> MEELLMSLKLKALYPLTGGYNRHSINPFYEELVRPTEIKGLWRWWNRVLFNTLAYSTKGKLYTYESIDRLFEDVFGSENKKSAVRLEVITDEGNDNRFELSYVELDKVIDCLRNYKRKVSLDFIDNTLIAEIEGSTKIPISFKSNLDIDKIIKDLVHNNKLLSFELLGFKSVEIDATKISDKKILKEILRDLITNYLEYFNIKQEVTFTLNIYLDKSREHKQNFEDKLKFALYSLLVFILLGGIGRKTSRGFGSLSIIDVKCYDNSICKKIEDLAKNFLKISSGNELKSKIESILDCIKNSCIDTLYIENNILSEIDPKKNVV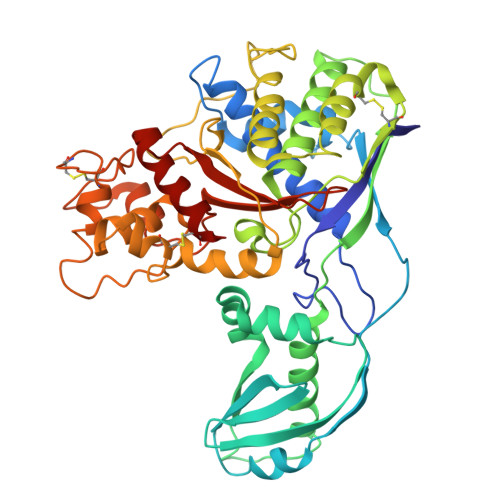YFINSDLFEVKRINDKEKVLANIYKAVSSEGCCIKSIITDKYVRKSFLIAFGGYRKVEKDKGLDIGFIKNYLCETCETVSSFNIVDFLLSEGSFMSDYILQYEHRNSLLRFKLISDNSNNSYLIGYILHSSYFKKIDIKYVRCILEKLTYCVI> KK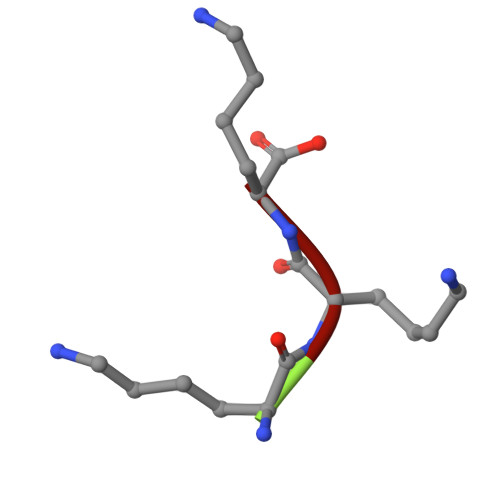K>MKILRGEEIAEKKAENLHGIIERSGLEPSLKLIQIGDNEAASIYARAKIRRGKKIGIAVDLEKYDDISMKDLLKRIDDLAKDPQINGIMIENPLPKGFDYYEIVRNIPYYKDVDALSPYNQGLIALNREFLVPATPRAVIDIMDYYGYHENTVTIVNRSPVVGRPLSMMLLNRNYTVSVCHSKTKDIGSMTRSSKIVVVAVGRPGFLNREMVTPGSVVIDVGINYVNDKVVGDANFEDLSEYVEAIT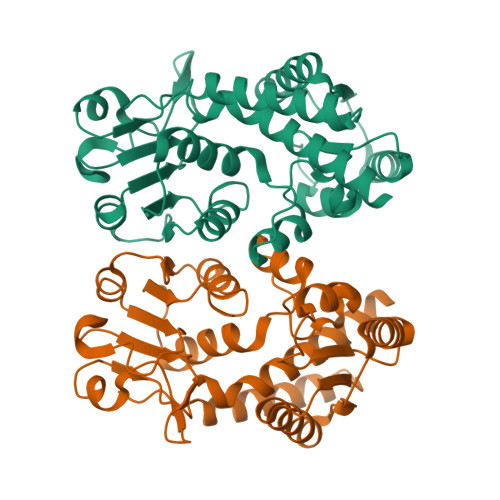PVPGGVGPITATNILENVVKAAEFQKNNL[2x]> GCGA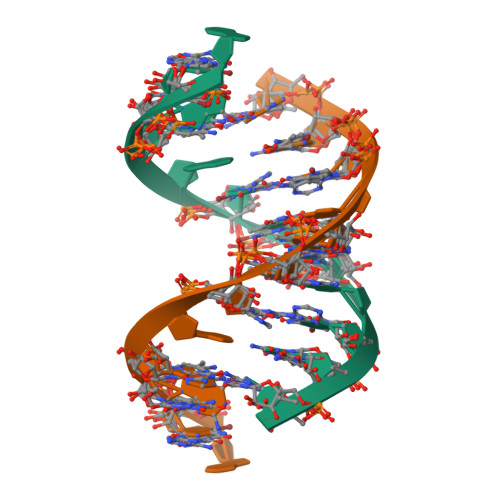AUTCGCGA>[2x]MTSLRDLIPKHKFDNSTIDQLCKLIDNEIEPIIFDLLKWLQDYNWPIAKDILPVVVLH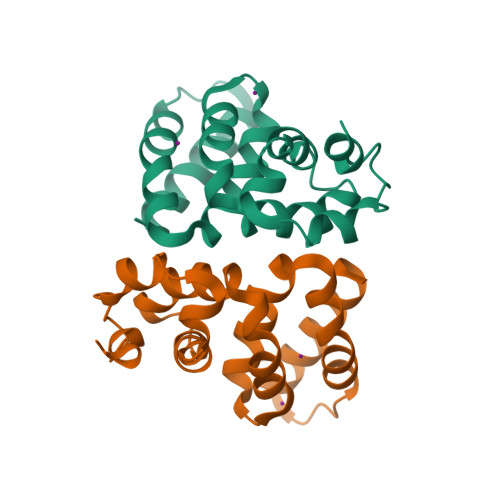QSIAMPHILTILQGNDIMWKYWVIKLMIPYLIYPNKQLVKSELERLSSLEIINEDIREIVNLSKDYLHFYYP>MSTSHVDDEDVNSIAVAKTDGLNQLYNLVAQDYALTDTIECLSRMLHRGTIPLDTFVKQGRELARQQFLVRWHIQRITSPLS[2x];>MAHHHHHHMQKHNIKLNQNQDISQLFHDEVPLFDNSITSKDKEVIETLSEIYSIVITLDHVEKAYLKDSIDDTQYTNTVDKLLKQFKVYLNSQNKEEINKHFQSIEAFCDTYNITASNAITRLERGIPITAEHAISTTTSAPSGDNKQSSSSDKK[2x];>[2x]MYVASWQDYHSDFSEKYGDIALKKKLEQNTKKLDEESSQLETTTRSIDS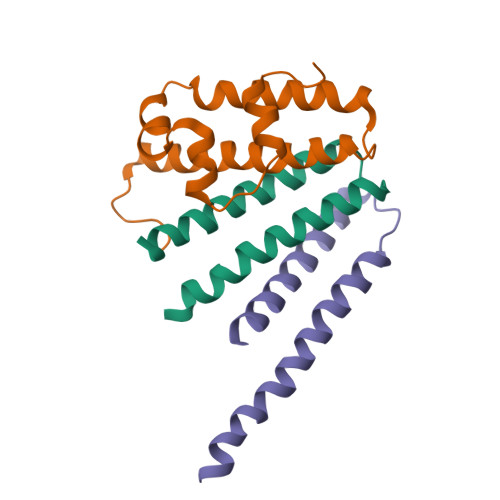ADDLDQFIKNYLDIRTQYHLRREKLATWDKQGNLKY>MHHHHHHGSGQRWELALGRFLEYLSWVSTLSEQVQEELLSSQVTQELRALMDETMKELKAYKSELEEQLTPVAEETRARLSKELQAAQARLGADMEDVRGRLVQYRGEVQAMLGQSTEELRVRLASHLIALQLRLIGDAFDLQKRLAVYQAGAAEQ[2x];>[2x]MAHAGRTGYDNREIVMKYI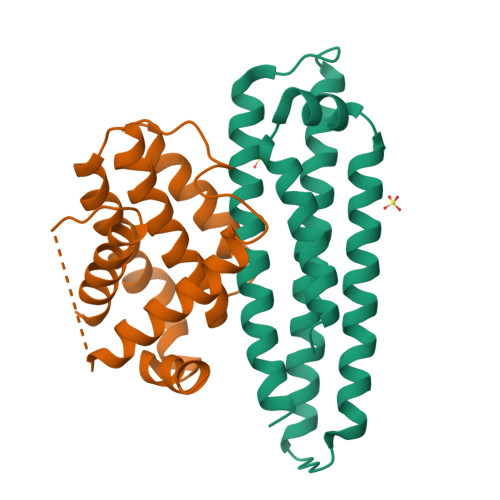HYKLSQRGYEWDAGDDVEENRTEAPEGTESEVVHLTLRQAGDDFSRRYRRDFAEMSSQLHLTPFTARGRFATVVEELFRDGVNWGRIVAFFEFGGVMCVESVNREMSPLVDNIALWMTEYLNRHLHTWIQDNGGWDAFVELYGPSMR Relative of Early Flowing 6 is a DNA-sequence-specific H3K27me3/2 demethylase that contains four zinc finger (ZnF) domains and targets several thousand genes in Arabidopsis thaliana. REF6 and ELF6 share a high sequence similarity comprising an N-terminal Jumonji N (JmjN) domain, a JmjC domain, and tandem zinc finger (ZnF) domains in the C-terminus. The ZnFs of REF6 are found to bind CTCTGYTY (where Y is C or T) DNA motifs directly and recognize specific nucleosomes. Here, we determined crystal structures of the ZnF domains and REF6-DNA complex, revealing a unique REF6-family-specific half-cross-braced ZnF (RCZ) domain and two C2H2-type ZnFs.

Attempts to cocrystallize REF6 (residues 1223–1360) with different lengths of dsDNA resulted in a complex crystal with a 15-bp DNA fragment (m5). The structure was solved to a resolution of 2.7 Å using the SAD method by SHELX C/D/E. In the asymmetric unit, one REF6, one dsDNA, two glycerol molecules, and 79 water molecules are modeled into the density map. Compared with holo-REF6, most of the acidic region is resolved in the complex structure. Direct binding with the dsDNA strand involves insertion of the ZnF3 and ZnF4 helices into the major groove. Surprisingly, only helices α3 and α4 insert into the DNA major groove. Helix α2 of the RCZ domain is situated above the major groove while helix α1 projects away from the DNA entirely. Conformations of the holo-REF6 and REF6-DNA binary complex differ greatly with an overall RMSD of 5.3 Å. Therefore, residues 1291–1293 act as a flexible hinge and dsDNA binding induces profound conformational changes of REF6. Structural observation showed that the DNA was bent by 16° compared with the standard B-form DNA duplex.

> GSVEEKEEEEEEEENEEEECAAYQCNMEGCTMSFSSEKQLMLHKRNICPIKGCGKNFFSHKYLVQHQRVHSDDRPLKCPWKGCKMTFKWAWSRTEHIRVHTGARPYVCAEPDCGQTFRFVSDFSRHKRKTGHSVKKTNKR> MVLQELWFGVIAALFLGFFILEGFDFGVGMLMAPFAHVGMGDPETHRRTALNTIGPVWDGNEVWLITAGAAIFAAFPGWYATVFSALYLPLLAILFGMILRAVAIEWRGKIDDPKWRTGADFGIAAGSWLPA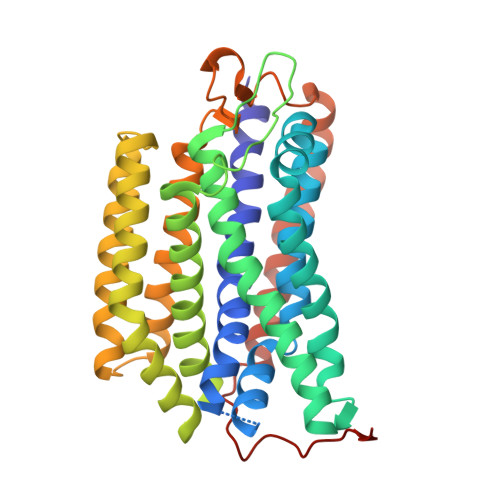LLWGVAFAILVRGLPVDANGHVALSIPDVLNAYTLLGGLATAGLFSLYGAVFIALKTSGPIRDDAYRFAVWLSLPVAGLVAGFGLWTQLAYGKDWTWLVLAVAGCAQAAATVLVWRRVSDGWAFMCTLIVVAAVVVLLFGALYPNLVPSTLNPQWSLTIHNASSTPYTLKIMTWVTAFFAPLTVAYQTWTYWVFRQRISAERIPPPTGLARRAP> SHMEGRLVVYCSATNAMCEAGTKAFAEKYNVNTSFVRNGSGSTLAKIDAEKNNPRADVWYGGTLDPQSQAGEMDLLQAYQSPELANIMEGFRDPAKRKGNYSSAVYMGILGFGVNTERLAQKGIPIPRCWADLTKPEYKGEIQISDPQSSGTAYTALATFIQLWDEPTAFEYFKKLDKNVSQYTKSG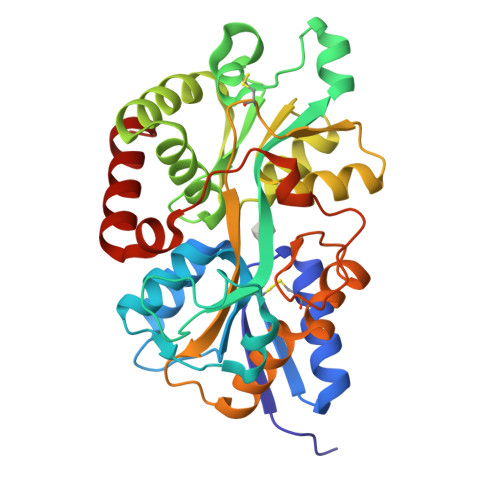VTPSRNSARGEVAIGIGFLHDYSLEQAKGAPLELISPCEGTGYELGGVSIIKGARNLDNAKLFVDWVLSKEGQEVAWKQGDSYQILTNTQAEQSPNALDPKTLKLINYDMETYGSSDERKRLITKWVNEIKMGN The removal of these introns is carried out by a conserved splicing machinery known as tRNA splicing endonuclease (EndA or TSEN). In archaea, four distinct types of EndAs that share similar architectural arrangements but employ different domains and subunit compositions are observed, including α4, α′2, (αβ)2, and ε2-type complexes, while the eukaryotic TSEN complex is a heterotetrametric complex consisting of four subunits: two structural units, TSEN15 and TSEN54, and two catalytic units, TSEN34 and TSEN2. TSEN54 and TSEN15 function as scaffolds to recruit the catalytic subunits TSEN34 and TSEN2. The C-terminal domains (CTD) of TSEN34 and TSEN2 contain the catalytic region and are arranged close to each other, which is the structural basis of the conserved recognition mechanism known as the ‘cross-subunit cation-π-sandwich’ pattern.

In this work, we report the structure of an active human tRNA splicing endonuclease complex bound to an intron-containing pre-tRNA, revealing the recognition and cleavage mechanism of pre-tRNA by human TSEN endonuclease complex. To obtain more homogeneous samples and capture the in-action structure of the wild-type complex, we reduced the incubation time, omitted the subsequent gel filtration step, and kept the sample at 4 °C or on ice, which preserved the integrity of most pre-tRNA molecules during the process of freezing the grid. This way helped minimize the cleavage reaction and allowed us to observe the pre-tRNA trapped in the endonuclease active site. The overall structural arrangement of the human TSEN complex is in a rectangular parallelepiped pattern, similar to that of the α′2-type endonuclease from Archaeglobus fulgidus bound with a BHB RNA. The conformation of the endonuclease-RNA complex observed here is poised for the cleavage reaction. The scissile phosphate is located at the center of the catalytic triad of residues in TSEN2, Y369, H377, and K416. The positively charged KRKRR motif in the N-terminal insertion of TSEN2, which is common in most eukaryotic TSEN2 but lacking in archaea, covers up the active site of TSEN2. Interestingly, the complex structure presented in this study differed from both the catalytic-dead state and the post-catalytic state. This is supported by the presence of G38 and the NTE loop of TSEN2, a critical feature missing in all other structural studies.

> MHHHHHHGSMEERGDSEPTPGCSGLGPGGVRGFGDGGGAPSWAPEDAWMGTHPKYLEMMELDIGDATQVYVAFLVYLDLMESKSWHEVNCVGLPELQLICLVGTEIEGEGLQTVVPTPITASLSHNRIREILKASRKLQGDPDLPMSFTLAIVESDSTIVYYKLTDGFMLPDPQNISLRR;> MAEAVFHAPKRKRRVYETYESPLPIPFGQDHGPLKEFKIFRAEMINNNVIVRNAEDIEQLYGKGYFGKGILSRSRPSFTISDPKLVAKWKDMKTNMPIITSKRYQHSVEWAAELMRRQGQDESTVRRILKDYTKPLEHPPVKRNEEAQVHDKLNSGMVSNMEGTAGGERPSVVNGDSGKSGGVGDPREPLGCLQEGSGCHPTTESFEKSVREDASPLPHVCCCKQDALILQRGLHHEDGSQHIGLLHPGDRGPDHEYVLVEEAECAMSEREAAPNEELVQRNRLICRRNPYRIFEYLQLSLEEAFFLVYALGCLSIYYEKEPLTIVKLWKAFTVVQPTFRTTYMAYHYFRSKGWVPKVGLKYGTDLLLYRKGPPFYHASYSVIIELVDDHFEGSLRRPLSWKSLAALSRVSVNVSKELMLCYLIKPSTMTDKEMESPECMKRIKVQEVILSRWVSSRERSDQDDL;> MLVVEVANGRSLVWGAEAVQALRERLGVGGRTVGALPRGPRQNSRLGLPLLLMPEEARLLAEIGAVTLVSAPRPDSRHHSLALTSFKRQQEESFQEQSALAAEARETRRQELLEKITEGQAAKKQKLEQASGASSSQEAGSSQAAKEDETSDGQASGEQEEAGPSSSQAGPSNGVAPLPRSALLVQLATARPRPVKARPLDWRVQSKDWPHAGRPAHELRYSIYRDLWERGFFLSAAGKFGGDFLVYPGDPLRFHAHYIAQCWAPEDTIPLQDLVAAGRLGTSVRKTLLLCSPQPDGKVVYTSLQWASLQ;> SYWDMEPEPEPAAVEVPAGRVLSARELFAARSRSQKLPQRSHGPKDFLPDGSAAQAERLRRCREELWQLLAEQRVERLGSLVAAEWRPEEGFVELKSPAGKFWQTMGFSEQGRQRLHPEEALYLLECGSIHLFHQDLPLSIQEAYQLLLTDHTVTFLQYQVFSHLKRLGYVVRRFQPSSVLSPYERQLNLDASVQHLEDGDGKRKRSSSSPRSINKKAKALDNSLQPKSLAASSPPPCSQPSQCPEEKPQESSPMKGPGGPFQLLGSLGPSPGPAREGVGCSWESGRAENGVTGAGKRRWNFEQISFPNMASDSRHTLLRAPAPELLPANVAGRETDAESWCQKLNQRKEKLSRREREHHAEAAQFQEDVNADPEVQRCSSWREYKELLQRRQVQRSQRRAPHLWGQPVTPLLSPGQASSPAVVLQHISVLQTTHLPDGGARLLEKSGGLEIIFDVYQADAVATFRKNNPGKPYARMCISGFDEPVPDLCSLKRLSYQSGDVPLIFALVDHGDISFYSFRDFTLPQDVGH>[2x]SMQRTVARDITLLECVGKGRYGEVWRGSWQGENVAVKIFSSRDEKSWFRETELYNTVMLRHENILGFIASDMTSRHSSTQLWLITHYHEMGSLYDYLQLTTLDTVSCLRIVLSIASGLAHLHIEIFGTQGK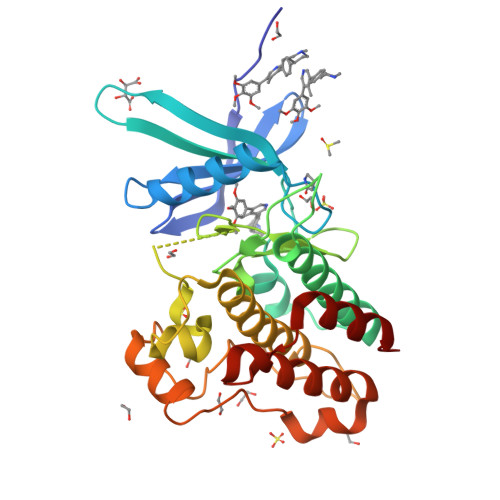PAIAHRDLKSKNILVKKNGQCCIADLGLAVMHSQSTNQLDVGNNPRVGTKRYMAPEVLDETIQVDCFDSYKRVDIWAFGLVLWEVARRMVSNGIVEDYKPPFYDVVPNDPSFEDMRKVVCVDQQRPNIPNRWFSDPTLTSLAKLMKECWYQNPSARLTALRIKKTLTKID> SSERIRYAKWMLEHGFNIIPIDPESKKPVLKEWQKYSHEMPSDEEKQRFLKMIEEGYNYAIPGGQKGMVIMDFESKEKLKAWIGESALEELCRKTLCTNTVHGGIHIYVLSNDIPPHKINPLFEENGKGIIDLQSYNSYVLGLGSCVNHLHCTTDKCPWKEQNYTTCYTLYNELKEISKVDLKSLLRFLAEKGKRLGITLSKTAKE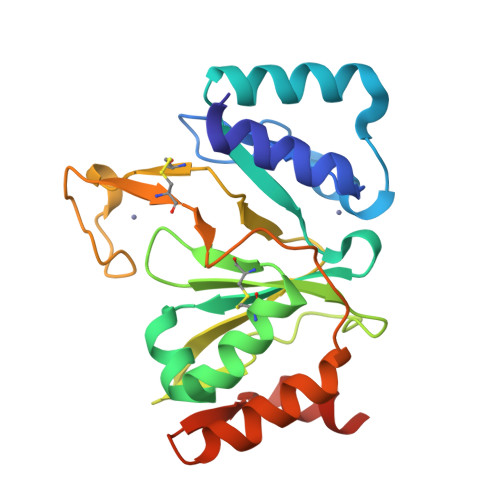WLEGHHHHHH> MAGNKPFNKQQAEPRERDPQVAGLKVPPHSIEAEQSVLGGLMLDNERWDDVAERVVADDFYTRPHRHIFTEMARLQESGSPIDLITLAESLERQGQLDSVGGCAYLAELSKNTPSAANISAYADIVRERAVVREMISVANEIAEAGFDPQGRTSEDLLDLAESRVFKIAESRANKDEGPKNIADVLDAT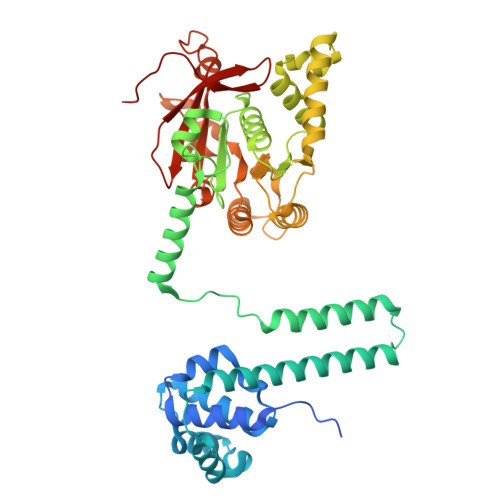VARIEQLFQQPHDGVTGVNTGYDDLNKKTAGLQPSDLIIVAARPSMGKTTFAMNLVENAAMLQDKPVLIFSLEMPSEQIMMRSLASLSRVDQTKIRTGQLDDEDWARISGTMGILLEKRNIYIDDSSGLTPTEVRSRARRIAREHGGIGLIMIDYLQLMRVPALSDNRTLEIAEISRSLKALAKELNVPVVALSQLNRSLEQRADKRPVNSDLRESGSIEQDADLIMFIYRDEVYHENSDLKGIAEIIIGKQRNGPIGTVRLTFNGQWSRFDNYAGPQYDDE>[10x]MAHHHHHHVDDDDKAAS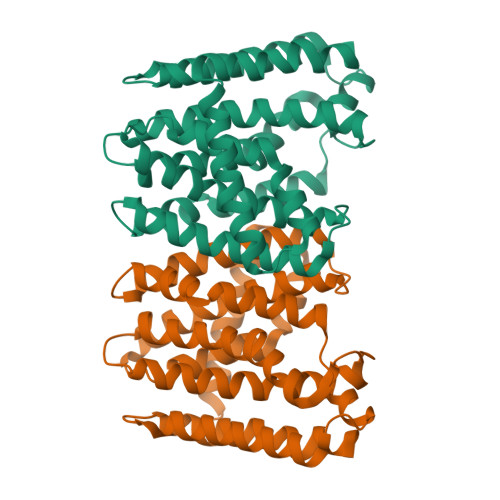WSHPQFEKGAENLYFQSMLAAEAANRDHVTRCVAQTGGSPDLVAHTAALRLYLRVPHFLTEWTTDPDRRAAVSRALALDIVSMKLLDDLMDDDTGLDRVELACVCLRLHLRALHELESLARDPKAVTDILEQDAVHLCGGQIRTKRSRATNLREWRAHASTYGSTFLGRYGALAAACGGEGQPADSVREFAEAFAMTITMADDLTDYDRNGERDGNLAHLMRTGAVAGQDVVDLLEELRGRALAAVAAPPGAPGLVPVVHLYTDDVLVRLLPRHLGE>[6x]MRTLLIRYILWRNDNDQTYYNDDFKKLMLLDELVDDGDVSTLIKNMRMTLSDGPLLDRLNYPVNNIEDAKRMIAISAKVA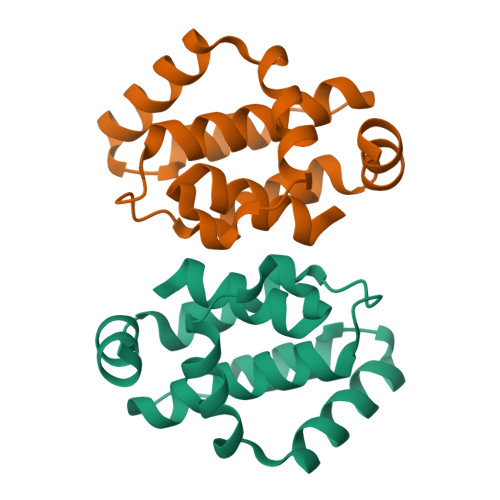RDIGERSEIRWEESFTILFRMIETYFDDLMIDLYGEKLEHHHHHH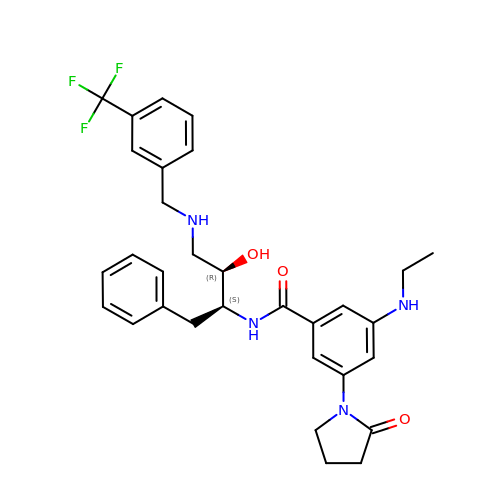N-[(1S,2R)-1-benzyl-2-hydroxy-3-{[3-(trifluoromethyl)benzyl]amino}propyl]-3-(ethylamino)-5-(2-oxopyrrolidin-1-yl)benzamide | C31 H35 F3 N4 O3 | QPGDTFHILHXFBQ-WUFINQPMSA-N>[2x]AQSVPYGISQIKAPA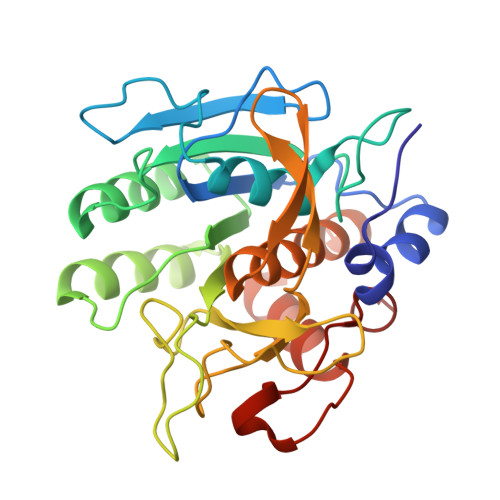LHSQGYTGSNVKVAVIDSGIDSSHPDLNVRGGASFVPSETNPYQDGSSHGTHVAGTIAALNNSIGVLGVAPSASLYAVKVLDSTGSGQYSWIINGIEWAISNNMDVINMSLGGPSGSTALKTVVDKAVSSGIVVAAAAGNEGSSGSTSTVGYPAKYPSTIAVGAVNSSNQRASFSSVGSELDVMAPGVSIQSTLPGGTYGAYNGTSMATPHVAGAAALILSKHPTWTNAQVRDRLESTATYLGNSFYYGKGLINVQAAAQ> ADYQGKNVVIIGLGLTGLSCVDFFLARGVTPRVMDTRMTPPGLDKLPEAVERHTGSLNDEWLMAADLIVASPGIALAHPSLSAAADAGIEIVGDIELFCREAQAPIVAITGSNGKSTVTTLVGEMAKAAGVNVGVGGNIGLPALMLLDDECELYVLELSSFQLETTSSLQAVAATILNVTEDHMDRYPFGLQQYRAAKLRIYENAKVCVVNADDALTMPIRGADERCVSFGVNMGDYHLNHQQGETWLRVKGEKVLNVKEMKLSGQHNYTNALAALALADAAGLPRASSLKALTTFTGLPHRFEVVLEHNGVRWINDSKATNVGSTEAALNGLHVDGTLHLLLGGDGKSADFSPLARYLNGDNVRLY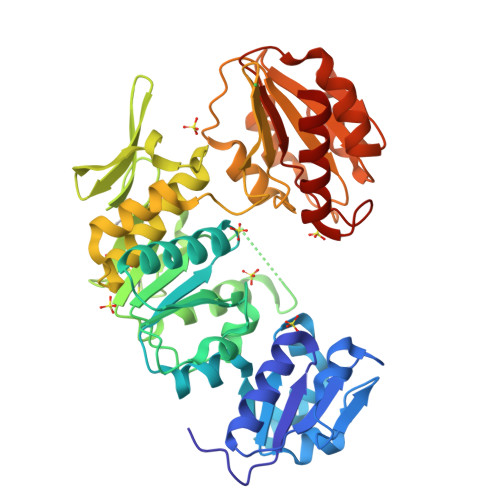CFGRDGAQLAALRPEVAEQTETMEQAMRLLAPRVQPGDMVLLSPACASLDQFKNFEQRGNEFARLAKELG N-{4-[(2-amino-4-hydroxy-7H-pyrrolo[2,3-d]pyrimidin-5-yl)methyl]benzoyl}-L-glutamic acid | C19 H19 N5 O6 | 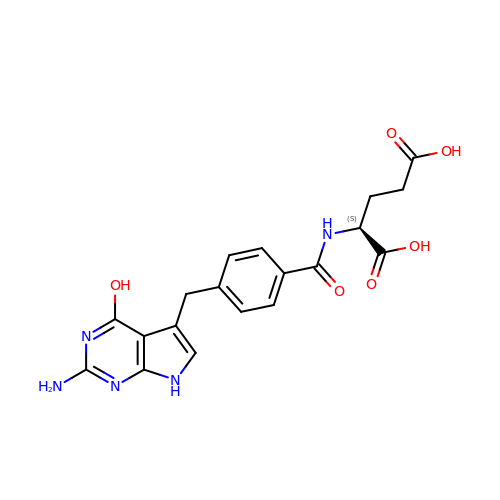VDHBMZRBPMTLGE-LBPRGKRZSA-N In this Trojan horse approach, the transport of drug conjugates is redirected via TonB-dependent receptors (TBDR), which are involved in the uptake of essential nutrients, including iron. By in silico screening, we further identified a PiuA orthologue, termed PiuD, present in clinical isolates, including strain LESB58. PiuD has a similar crystal structure as PiuA and is involved in the transport of the siderophore-drug conjugates BAL30072, MC-1, and cefiderocol in strain LESB58. An in silico screen identified PiuD in LESB58 and other clinical isolates as a homologue of PiuA, sharing 60% amino acid identity.

Here, we determined the structure of PiuD from strain 39016, which shows 99.6% amino acid identity with PiuD (PALES_48941) from LESB58. The obtained PiuD structure was similar to that of PiuA from PAO1. The crystallographic asymmetric unit has two monomers (denoted A and B). PiuD comprised two domains, a 22-stranded transmembrane β-barrel and an N-terminal plug domain (residues 27 to 156) folded inside the barrel. The plug domain has two β-sheets and two α-helices, which together, occluded the central pore. As often occurs in the TBDR structures, some of the extracellular loops were not experimentally located in the PiuD structure. In the B monomer, these regions, namely, NL1 (83 and 84), NL3 (113 and 114), the loop 138 to 141 of the plug domain, L7 (504 to 530), L8 (564 to 572), and L9 (609 to 624), were presumed to be disordered. As a consequence of the disorder, one side of the extracellular β-barrel was absent. The closest structural relatives were PiuA of A. baumannii (root mean square deviation [RMSD] of 1.1 Å over 701 residues) and P. aeruginosa (1.1 Å over 656 residues) and the pyochelin receptor FptA from P. aeruginosa (1.8 Å over 655 residues). Like PiuA, PiuD also has a distinctive cluster of aromatic and positively charged residues located inside the pore at the extracellular face.

>[2x]AMNEAGQKKTDKDRVLSLDAATIVGEQQDETTYNVDRSASKKYTAPLLDTPRSVTVVPKQVIKDTAAVSLQDALRTVPGITFGAGEGGNPTGDRPFIRGFDAQSDTYVDGVRDTGAQTREIFNLEQIEVSKGPNSAFGGRGSAGGSLNLVSKQAKAGNFIDGGFTYGSDQTRRYTLDLNQEFLDGNAAFRLNLLKHDANVAGRDEVDVSRWGVAPSLTFGLGSPTRVTVSHYHLESDDTPDSGIPYAKSSDRSKHNPDKPVNVDRGNFYGLTGRDFQKSRIDTSTITVEHDLTDSLTIRNTSRYGNSHQDYLWTQPDDSQGNINNGSVWRRQNNRVSTTTTAVNQTDLFGEFYLGGFKNSFSTGLEFSREDSKRDGYIVDTNTGLGSNKCNPSLIGAPSGYNCTSLENPNPHDPWNGSITRKYAPLNTVGTTKAIYAFDTIDLNEQWQVNIGARFDSFETTAKNHGVRPATKLSDKSSFWNWQAGLVWKPVPNGSIYASYATSATPPGSMLDNGDTSNAVDGFAISNNLEPEETTNYELGTKWAFFNERLELSAAIFRTDKDNTRILVANQTYDNAGQSRVDGVELSASGKLTEKWKVFAGYSYLDSELVDAGKAGRNGNVNASAASNNGNEMPNTPKNSFSLWTTYDIFPKTTIGGGAFYVDKVYGDVGNTVYVPDYWRYDAMASYKLSKNVDFQLNVQNVFDKKYFDKAYAAHYASQAAGRTILFSTNFHFLEHHHHHH> GPDSMAAGFKTVEPL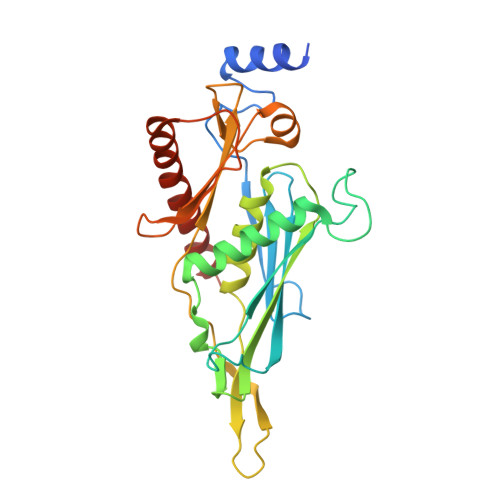EYYRRFLKENCRPDGRELGEFRTTTVNIGSISTADGSALVKLGNTTVICGVKAEFAAPSTDAPDKGYVVPNVDLPPLCSSRFRSGPPGEEAQVASQFIADVIENSQIIQKEDLCISPGKLVWVLYCDLICLDYDGNILDACTFALLAALKNVQLPEVTINEETALAEVNLKKKSYLNIRTHPVATSFAVFDDTLLIVDPTGEEEHLATGTLTIVMDEEGKLCCLHKPGGSGLTGAKLQDCMSRAVTRHKEVKKLMDEVIKSMKPK>[6x]MSITLRTYI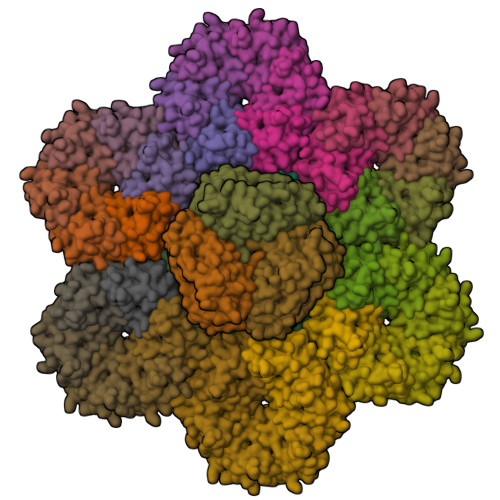FLDALQPQLATFIGKTARGFLPVPGQASLWVEIAPGIAINRVTDAALKATKVQPAVQVVERAYGLLEVHHFDQGEVLAAGSTILDKLEVREEGRLKPQVMTHQIIRAVEAYQTQIINRNSQGMMILPGESLFILETQPAGYAVLAANEAEKAANVHLVNVTPYGAFGRLYLAGSEAEIDAAAEAAEAAIRSVSGVA;>MADALGMIEVRGFVGMVEAADAMVKAAKVELIGYEKTGGGYVTAVVRGDVAAVKAATEAGQRAAERVGEVVAVHVIPRPHVNVDAALPLGRTPGMDKSA[36x]>[12x]MAKRIKNTTPKQDGFRMPGEFEKQKQIWMLWPWRNDNWRLGAKPAQKAFLEVAE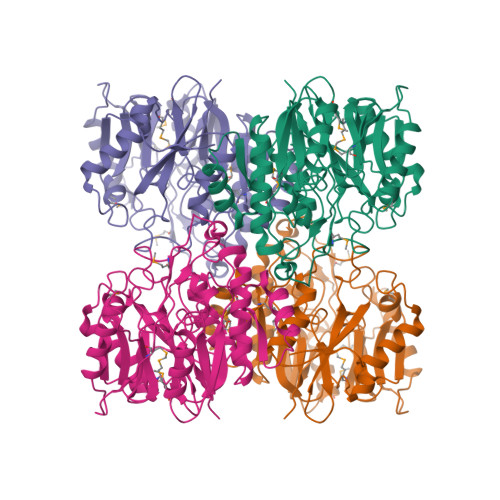AISEFEPVSLCVPPLQYENALARVSELGSHNIRIIEMTNDDAWIRDCGPTFLVNDKGDLRAVDWEFNAWGGLVDGLYFPWDQDALVARKVCEIEGVDSYKTKDFVLEGGSIHVDGEGTVLVTEMCLLHPSRNPHLTKEDIEDKLKDYLNCVKVLWVKDGIDPYETNGHIDDVACFIRPGEVACIYTDDKEHPFYQEAKAAYDFLSQQTDAKGRPLKVHKMCVTKEPCYLQEAATIDYVEGSIPREEGEMAIASYLNFLIVNGGIILPQYGDENDQLAKQQVQEMFPDRKVVGVRTEEIAYGGGNIHCITQQQPATLEHHHHHH>MGSSHHHHHHSSGNEIKLILQQYLEKFEAHYERVLQDDQYIEALETLMDDYSEFILNPIYEQQFNAWRDVEEKAQLIKSLQYITAQCVKQVEVIRARRLLDGQASTTGYFDNIEHCIDEEFGQCSITSNDKLLLVGSGAYPMTLIQV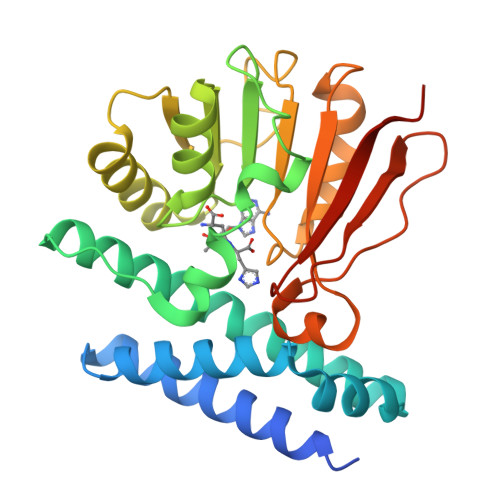AKETGASVIGIDIDPQAVDLGRRIVNVLAPNEDITITDQKVSELKDIKDVTHIIFSSTIPLKYSILEELYDLTNENVVVAMRFGDGIKAIFNYPSQETAEDKWQCVNKHMRPQQIFDIALYKKAAIKVGITD[4x]> SLFEAWAKPVQPFAIWPGVWYVGTENLSSVLLT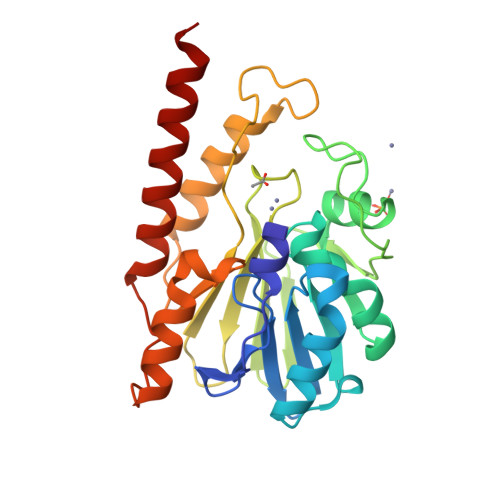TPQGHILIDAGLDASAPQIRRNIEALGFRMADIRYIANSHARLDHAGGIARLKAWSGARVIASHANAEQMARGGKEDFALGDALPFPPVTVDMEAQDGQQWHLGGVTLAAIFTPGHLPGATSWKVTLADGKTLIYADSLATPGYPLINNRNYPTLVEDIRRSFARLEAQQVDIFLANHGERFGLMDKMARKARGENNAFIDKAGLARYVAQSRAAFEKQLAAQRAQP> ASKVYDPEQRKRMITGPQWWARCKQMNVLDSFINYYDSEKHAENAVIFLHGNATSSYLWRHVVPHIEPVARCIIPDLIGMGKSGKSGNGSYRLLDHYKYLTAWFELLNLPKKIIFVGHDWGAALAFHYAYEHQDRIKAIVHMESVVDVIESWDEW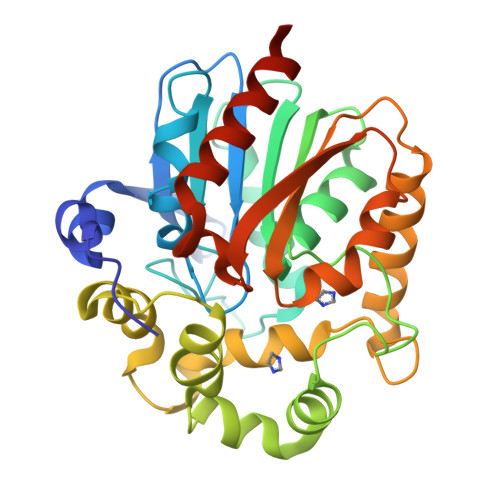PDIEEDIALIKSEEGEKMVLENNFFVETVLPSKIMRKLEPEEFAAYLEPFKEKGEVRRPTLSWPREIPLVKGGKPDVVQIVRNYNAYLRASDDLPKLFIESDPGFFSNAIVEGAKKFPNTEFVKVKGLHFLQEDAPDEMGKYIKSFVERVLKNEQVDHHHHHH>SQGHKPLEVIKIEDGVYLHTSFKNIEGYGLVDSNGLVVLDNNQAYIIDTPWSEEDTKLLLSWATDRGYQVMASISTHSHEDRTAGIKLLNSKSIPTYTSELTKKLLAREGKPVPTHYFKDDEFTLGNGLIELYYPGAGHTEDNIVAWLPKSKILFGGCLVRSHEWEGLGYVGDASISSWADSIKNIVSKKYPIQMVVPGHGKVGSSDILDHTIDLAESASNKLMQPTAEASAD[2x];> SQGHKPLEVIKIEDGVYLHTSFKNIEGYGLVDSNGLVVLDNNQAYIIDTPWSEEDTKLLLSWATDRGYQVMASISTHSHEDRTAGIKLLNSKSIPTYTSELTKKLLAREGKPVPTHYFKDDEFTLGNGLIELYYPGAGHTEDNIVAWLPKSKILFGGCLVRSHEWEALGYVGDASISSWADSIKNIVSKKYPIQMVVPGHGKVGSSDI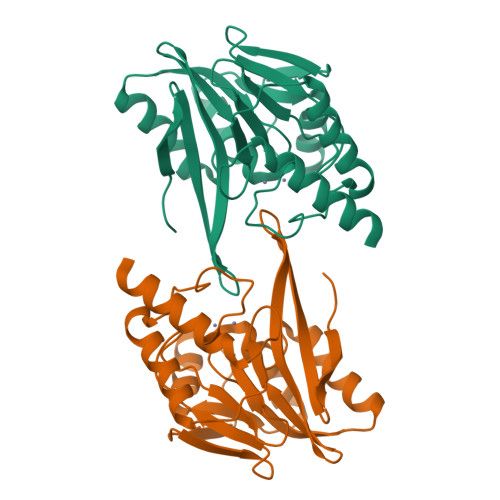LDHTIDLAESASNKLMQPTAEASAD>MPCSCASGCQKSKNGGSTPSIRDHVADYYGKTLQSSADLKTSACKLAAAVPESHRKILADIADEVLEKFYGCGSTLPADGSLEGATVLDLGCGTGRDVYLASKLVGEHGKVIGVDMLDNQLEVARKYVEYHAEKFFGSPSRSNVRFLKGFIENLATAEPEGVPDSSVDIVISNCVCNLSTNKLALFKEIHRVLRDGGELYFSDVYADRRLSEAAQQDPILYGECLGGALYLEDFRRLVAEAGFRDVRLVSVGPVDVS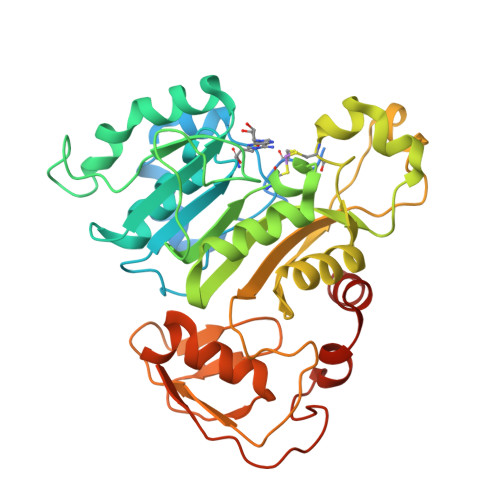DPQLRKLVPDVQFYSCTFRCFKVATLEATREDYGQSATYLGGIGEEFKLDRFFTFPREKPVRVDRNTAEIIRHSRLHQWFSVSAEQQHMGLFKANDSYALLHAPLSMQVEQLVSHHHHHH[2x]>MGSSHHHHHHSGLVPRGSHMATPPKRSSPSFSASSEGTRIKKISIEGNIAAGKSTFVNILKQLSEDWEVVPEPVARWSNVQSTQDEFEELTMEQKNGGNVLQMMYEKPERWSFTFQTY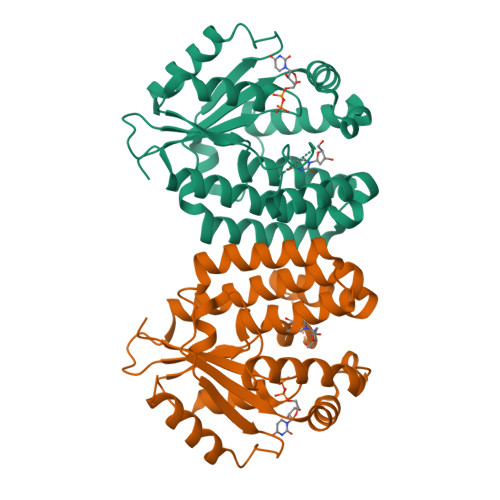ACLSMIRAQLASLNGKLKDAEKPVLFFERSVYSARYIFASNLYESESMNETEWTIYQDWHDWMNNQFGQSLELDGIIYLQATPETCLHRIYLRGRNEEQGIPLEYLEKLHYKHESWLLHRTLKTNFDYLQEVPILTLDVNEDFKDKYESLVEKVKEFLSTL[2x]>MGRSHHHHHHGSLVPRGSEQGSNVNHLIKVTDQSITEGYDDSDGIIKAHDAENLIYDVTFEVDDKVKSGDTMTVNIDKNTVPSDLTDSFAIPKIKDNSGEIIATGTYDNTNKQITYTFTDYVDKYENIKAHLKLTSYIDKSKVPNNNTKLDVEYKTALSSVNKTITVEYQKPNENRTANLQSMFTNIDTKNHTVEQTIYINPLRYSAKETNVNISGNGDEGSTIIDDSTIIKVYKVGDNQNLPDSNRIYDYSEYEDVTND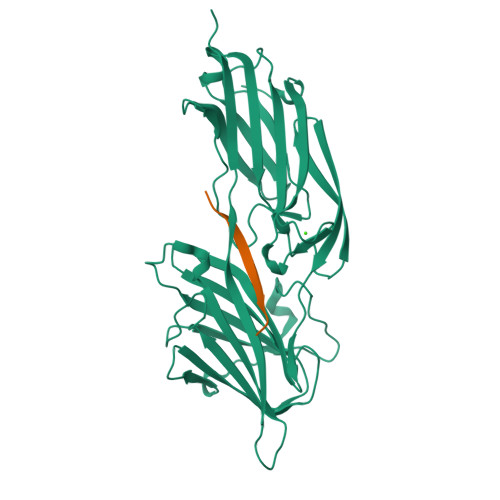DYAQLGNNNDVNINFGNIDSPYIIKVISKYDPNKDDYTTIQQTVTMQTTINEYTGEFRTASYDNTIAFSTSSGQGQGDLPPEK[2x];>NEEGFFFSARGHRPLD[2x]> SMGIVEEAHNLRVVGEGKRGVIVLAHGFGTDQSVWKHLVPHLVADYRVVLFDTMGAGPTNPDYFDFSRYATLEGYALDLL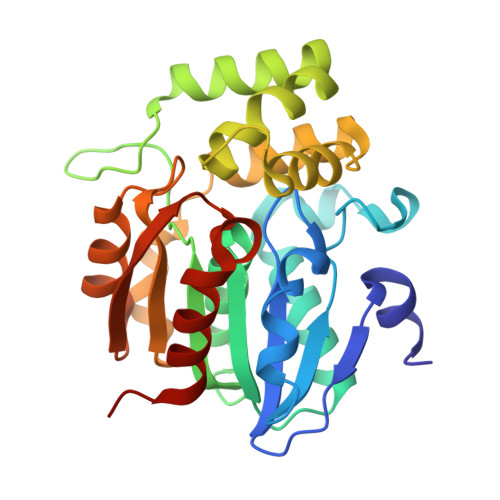AILQELRVASCIYVGHSVSAVIGAIASISRPDLFSKLVLLSASPRYLNDVDYYGGFEQEDLDELFEAMGSNYKAWCSGFAPLCVGGDMESVAVQEFSRTLFNIRPDIALSVAQTIFQSDVRSLLPLVTVPCHIVQSTKDLAVPVVVSEYLHKHLGGDSIVEVMPSEGHLPQLSSPDIVIPVLLRHIQHDIAV>[2x]GSVPATLPQLTPTLVSLLEVIEPEVLYAGYDSS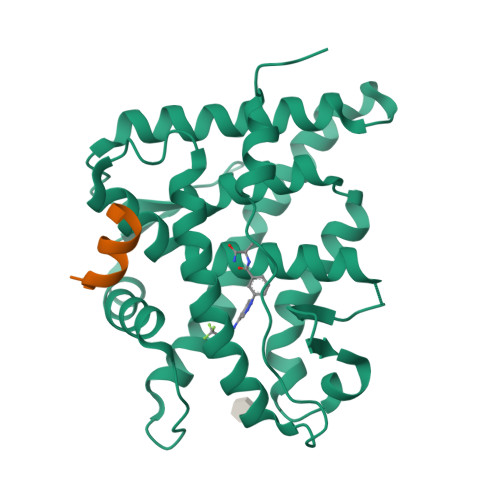VPDSTWRIMTTLNMLGGRQVIAAVKWAKAIPGFRNLHLDDQMTLLQYSWMYLMAFALGWRSYRQSSANLLCFAPDLIINEQRMTLPGMYDQCKHMLYVSSELHRLQVSYEEYLCMKTLLLLSSVPKDGLKSQELFDEIRMTYIKELGKAIVKREGNSSQNWQRFYQLTKLLDSMHEVVENLLNYCFQTFLDKTMSIEFPEMLAEIITNQIPKYSNGNIKKLLFHQK;>KENALLRYLLDK[2x]> GUUCUUA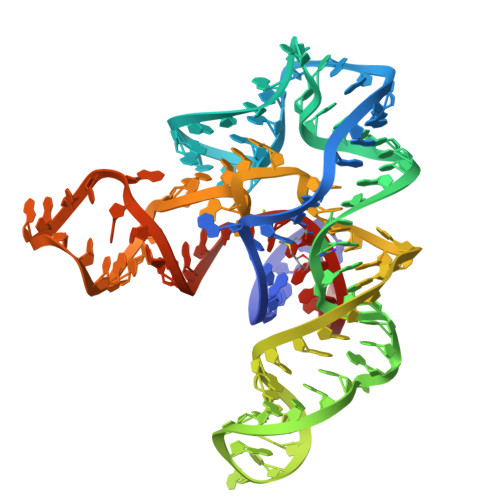UCAAGAGAAGCAGAGGGACUGGCCCGACGAAGCUUCAGCAACCGGUGUAAUGGCGAAAGCCAUGACCAAGGUGCUAAAUCCAGCAAGCUCGAACAGCUUGGAAGAUAAGAAC GAMMA-L-GLUTAMIC ACID | C5 H9 N O4 | 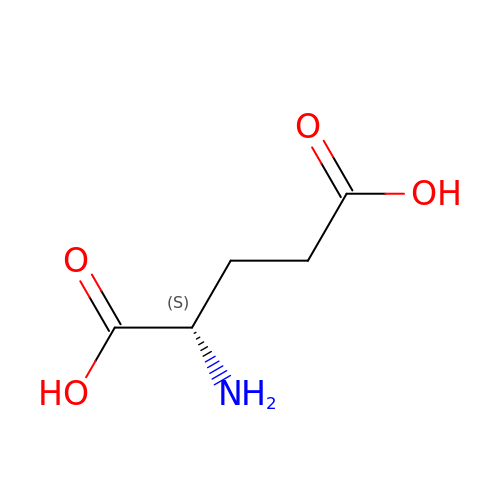WHUUTDBJXJRKMK-VKHMYHEASA-N> EEKEQKLQFVLRFGDFEDVISLSKLNVNGSKTTLYS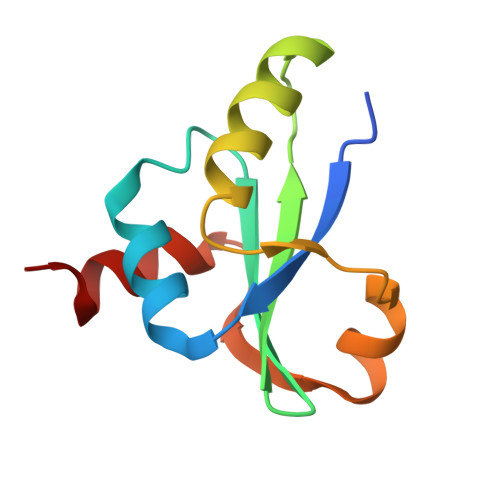FENRYYLYVDFCNMTDEEVENQLSILLEYATESSISIHRLEEYGKLIISEHALETIKKHFAS>[2x]MLNTTFANAKFANPFMNASGVHCMTIEDLEELKASQAGAYITKSSTLEKREGNPLPRYVDLELGSIN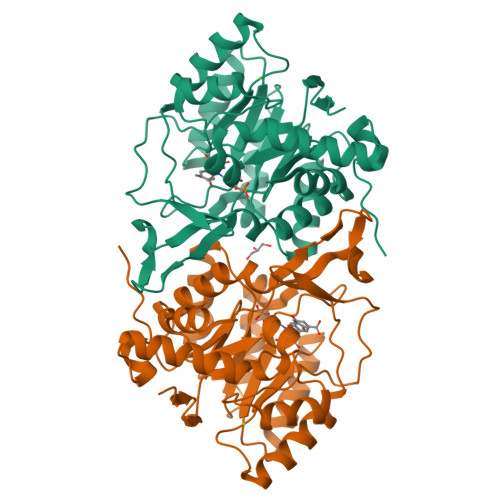SMGLPNLGFDYYLDYVLKNQKENAQEGPIFFSIAGMSAAENIAMLKKIQESDFSGITELNLSCPNVPGKPQLAYDFEATEKLLKEVFTFFTKPLGVKLPPYFDLVHFDIMAEILNQFPLTYVNSVNSIGNGLFIDPEAESVVIKPKDGFGGIGGAYIKPTALANVRAFYTRLKPEIQIIGTGGIETGQDAFEHLLCGATMLQIGTALHKEGPAIFDRIIKELEEIMNQKGYQSIADFHGKLKSL> MLHLLALFLHCLPLASGDYDICKSWVTTDEGPTWEFYACQPKVMRLKDYVKVKVEPSGITCGDPPERFCSHENPYLCSNECDASNPDLAHPPRLMFDKEEEGLATYWQSITWSRYPSPLEANITLSWNKTVELTDDVVMTFEYGRPTVMVLEKSLDNGRTWQPYQFYAEDCMEAFGMSARRARDMSSSSAHRVLCTEEYSRWAGSKKEKHVRFEVRDRFAIFAGPDLRNMDNLYTRLESAK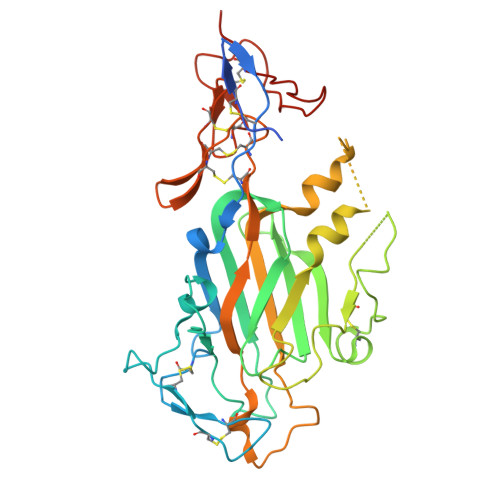GLKEFFTLTDLRMRLLRPALGGTYVQRENLYKYFYAISNIEVIGRCKCNLHANLCSMREGSLQCECEHNTTGPDCGKCKKNFRTRSWRAGSYLPLPHGSPNACAGTHHHHHH>[8x]MCTGVRFSDDEGNTYFGRNLDWSFSYGETILVTPRGYHYDTVFGAGGKAKPNAVIGVGVVMADRPMYFDCANEHGLAIAGLNFPGYASFVHEPVEGTENVATFEFPLWVARNFDSVDEVEETLRNVTLVSQIVPGQQESLLHWFIGDGKRSIVVEQMADGMHVHHDDV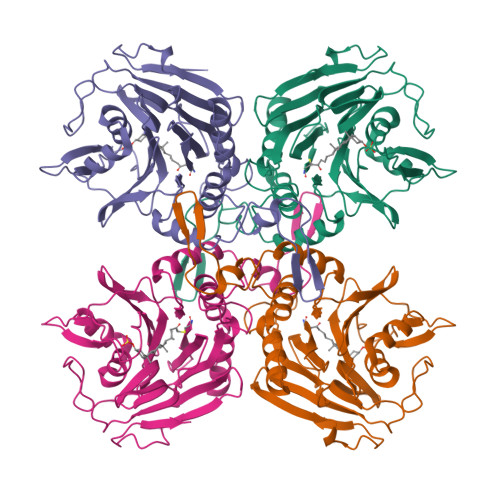DVLTNQPTFDFHMENLRNYMCVSNEMAEPTSWGKASLTAWGAGVGMHGIPGDVSSPSRFVRVAYTNAHYPQQNDEAANVSRLFHTLGSVQMVDGMAKMGDGQFERTLFTSGYSSKTNTYYMNTYDDPAIRSYAMADYDMDSSELISVAR> PAGIIPTGNVLSTIEVCAHRCIFDFFKQIRSDDNSLYSAQFDILLGTYCNTLNFVRFLELGLSVACICTKFPELAYVRDGVIQFEVQQPMIARDGPHPVDQPVHNYMVKRIHKRSLSAAFAIASEALSLLSNTYVDGTEIDSSLRIRAIQQMARNLRTVLDSFERGTADQLLGVLLEKAPPLSLLSPINKFQPEGHLNRVARAALLSDLKRRVCADMFFMTRHAREPRLISAYLSDMVSCTQPSVMVSRITHTNTRGRQVDGVLVTTATLKRQLLQGILQIDDTAADVPVTVLNGANLVTALVMGKAVRSLDDVGRHLLDMQEEQLENARVPADLVIVGDKLVFLEALERRVYQATRVAYPLIGNIDITFIMPMGVFQANSMDRYTRHAGDFSTVSEQDPRQFPPQGIFFYNKDGILTQLTLRDAMGTICHSSLLDVEATLVALRQQHLDRQCYFGVYVAEGTEDTLDVQMGRFMETWADMMPHHPHWVNEHLTILQFIAPSNPRLRFELNPAFDFFVAPGDVDLPGPQRPPEAMPTVNATLRIINGNIPVPLCPISFRDCRGTQLGLGRHTMTPATIKAVKDTFEDRAYPTIFYMLEAVIHGNERNFCALLRLLTQCIRGYWEQSHRVAFVNNFHMLMYITTYLGNGELPEVCINIYRDLLQHVRALRQTITDFTIQGEGHNGETSEALNNILTDDTFIAPILWDCDALIYRDEAARDRLPAIRVSGRNGYQALHFVDMAGHNFQRRDNVLIHGRPVRGDTGQAIPITPHHDREWGILSKIYYYIVIPAFSRGSCCTMGVRYDRLYPALQAVIVPEIPADEEAPTTPEDPRHPLHAHQLVPNSLNVYFHNAHLTVDGDALLTLQELMGDMAERTTAILVSSAPDAGAATATTRNMRIYDGALYHGLIMMAYQAYDETIATGTFFYPVPVNPLFACPEHLASLRGMTNARRVLAKMVPPIPPFLGANHHATIRQPVAYHVTHSKSDFNTLTYSLLGGYFKFTPISLTHQLRTGFHPGIAFTVVRQDRFATEQLLYAERASESYFVGQIQVHHHDAIGGVNFTLTQPRAHVDLGVGYTAVCATAALRCPLTDMGNTAQNLFFSRGGVPMLHDNVTESLRRITASGGRLNPTEPLPIFGGLRPATSAGIARGQASVCEFVAMPV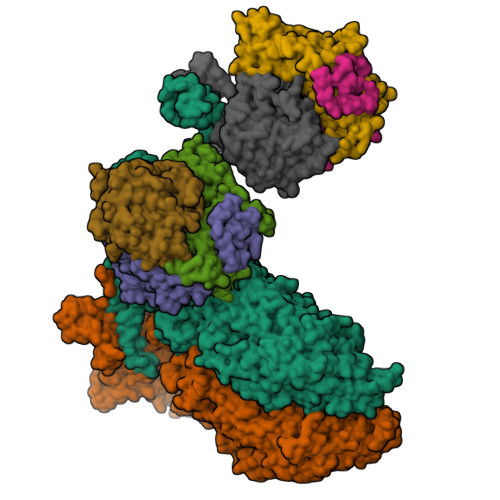STDLQYFRTACNPRGRASGMLYMGDRDADIEAIMFDHTQSDVAYTDRATLNPWASQKHSYGDRLYNGTYNLTGASPIYSPCFKFFTPAEVNTNCNTLDRLLMEAKAVASQSSTDTEYQFKRPPGSTEMTQDPCGLFQEAYPPLCSSDAAMLRTAHAGETGADEVHLAQYLIRDASPLRGCLPL;> IPAGIIPTGNVLSTIEVCIFFRFLELGLSVACICTKFPELAYVRDGVIQFEVQQPMIARDGPHPVDQPVHNYMVKRIHKRSLSAAFAIASEALSLLSNTYVDGTEIDSSLRIRAIQQMARNLRTVSDSFERGTADQLLGVLLEKAPPLSLLSPINKFQPEGHLNRVARAALLSDLKRRVCADMFFMTRHAREPRLISAYLSDMVSCTQPSVMVSRITHTNTRGRQVDGVLVTTATLKRQLLQGILQIDDTAADVPVTYGEMVLQGTNLVTALVMGKAVRNARVPADLVIVGDKLVFLEALERRVYQATRVAYPLIGNIDITFIMPMGVFQANSMDRYTRHAGDFSTVSEQDPRQFPPQGIFFYNKDGILTQLTLRDAMGTICHSSLLDVEATLVALRQQHLDRQCYFGVYVAEGTEDTLDVQMGRFMETWADMMPHHPHWVNEHLTILQFIAPSNPRLRFELNPAFDFFVAPGDVDLPGPQRPPEAMPTVNATLRIINGNIPVPLCPISFRDCRGTQLGLGRHTMTPATIKAVKDTFEDRAYPTIFYMLEAVIHGNERNFCALLRLLTQCIRGYWEQSHRVAFVNNFHMLMYITTYLGNGELPEVCINIYRDLLQHVRALRQTITDFTIQGEGHNGETSEALNNILTDDTFIAPILWDCDALIYRDEAARDRLPAIRVSGRNGYQALHFVDMAGHNFQRRDNVLIHGRPVRGDTGQAIPITPHHDREWGILSKIYYYIVIPAFSRGSCCTMGVRYDRLYPALQAVIVPEIPADEEAPTTPEDPRHPLHAHQLVPNSLNVYFHNAHLTVDGDALLTLQELMGDMAERTTAILVSSAPDAGAATATTRNMRIYDGALYHGLIMMAYQAYDETIATGTFFYPVPVNPLFACPEHLASLRGMTNARRVLAKMVPPIPPFLGANHHATIRQPVAYHVTHSKSDFNTLTYSLLGGYFKFTPISLTHQLRTGFHPGIAFTVVRQDRFATEQLLYAERASESYFVGQIQVHHHDAIGGVNFTLTQPRAHVDLGVGYTAVCATAALRCPLTDMGNTAQNLFFSRGGVPMLHDNVTESLRRITASGGRLNPTEPLPIFGGLRPATSAGIARGQASVCEFVAMPVSTDLQYFRTACNPRGRASGMLYMGDRDADIEAIMFDHTQSDVAYTDRATLNPWASQKHSYGDRLYNGTYNLTGASPIYSPCFKFFTPAEVNTNCNTLDRLLMEAKAVASQSSTDTEYQFKRPPGSTEMTQDPCGLFQEAYPPLCSSDAAMLRTAHAGETGADEVHLAQYLIRDASPLRGCLPL;>[2x]AMPFEIEVLLPGELSPAETSALQKCEGKIITFSTLRHRASLVDIALSSYYINGAPPDTLSLLEAYRMRFAAVITRVIPGKLLAHAIGVGTPTPGLFIQNTSPVDLCNGDYICLLPPVFGSADSIRLDSVGLEIVFPLTIPQTLMREIIAKVVARAVEDLNPDPDLNVLYYNGARLSLVADVQQLASDAAIRTLVLNLMFSINEGCLLILALIPRLLALGYVNALLQMQSVTREAAQLIHPEAPMLMRRLPIYETISSWISTSSRLGDTLGTRAILRVCVFDGPSTVHPGDRTAVIQV;>AMPFEIEVLLPGEISPAETSALQKCEGKIITFSTLRHRASLVDIALSSYYINGAPPDTLSLLEAYRMRFAAVITRVIPGKLLAHAIGVGTPTPGLFIQNTSPVDLCNGDYICLLPPVFGSADEIRLDSVGLEIVFPLTIPQTLMREIIAKVVARAVERTAAGRTPGELPGADVICYNGRRYELETNLQHRDGSDAAIRTLVLNLMFSINEGTTLILTLITRLLVQGAHDGYVNLLIQTANCVRETGQPMPRIQDGHRRFPIYEAISSWISTSSRLGDTLGTRAILRVCVFDGPSTVHPGDRTAVIQV[2x];>AAAAAAAAAAAAAAAAAAAAAAAAAAAAAAAAAAAAAIVINRMNNIQINPTSIGNPQTIRLPLNNFKSTTQLIQQVSLTDFFRPDIEHAGSTVLILRHPTDLPHLARHRAPPGRQTERLAEAWGQLLEASESGCARAYVTSLSFIAACRAEEYTDKQAAEANRTAIVSAYGCSRMGARLIRFSECLRAMVQCHVFPHRFISFFGSLLEYTIQDNLCNITAVAKGPQEAARTDKTSTRRVTANIPACVFWDVDKDLHLSADGLKHVFLVFVYTQRRQREGVRLHLALSQLNEQCFGRGIGFLLGARICMYAAYTLIGTIPSESVRYTRRMERFGGYNVPTIWLEGVVWGGTNTWNECY[2x]>[2x]KILPHRYPFLLVDKVIYMQPNKTIIGLKQVSTNEPFFNG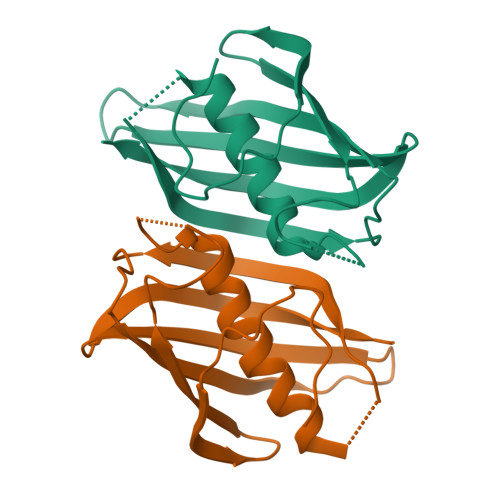HFPQKQIMPGVLQIEALAQLAGILCLKSDDSQKNNLFLFAGVDGVRWKKPVLPGDTLTMQANLISFKSSLGIAKLSGVGYVNGKVVINISEMTFALS>GSHMYLSKQLCFLFYVSSKEIIKKYTNYLKEYDLTYTGYIVLMAIENDEKLNIKKLGERVFLDSGTLTPLLKKLEKKDYVVRTREEKDERNLQISLTEQGKAIKSPLAEISVKVFNEFNISEREASDIINNLRNFVS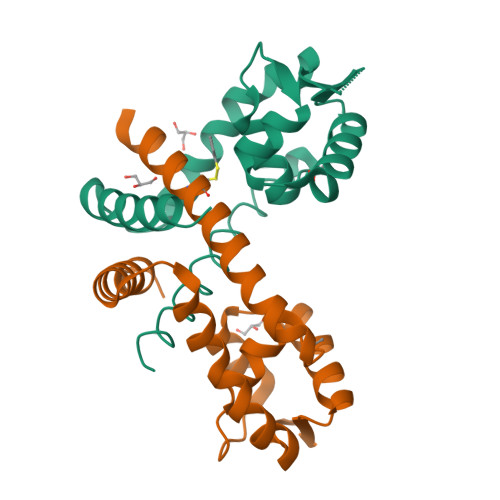KNF[4x]> ADEEQVFHFYWLDAYEDQYNQPGVVFLFGKVWIESAETHVSCCVMVKNIERTLYFLPREMKIDLNTGKETGTPISMKDVYEEFDEKIATKYKIMKFKSKPVEKNYAFEIPDVPEKSEYLEVKYSAEMPQLPQDLKGETFSHVFGTNTSSLELFLMNRKIKGPCWLEVKSPQLLNQPVSWCKAEAMALKPDLVNVIKDVSPPPLVVMAFSMKTMQNAKNHQNEIIAMAALVHHSFALDKAAPKPPFQSHFCVVSKPKDCIFPYAFKEVIEKKNVKVEVAATERTLLGFFLAKVHKIDPDIIVGHNIYGFELEVLLQRINVCKAPHWSKIGRLKRSNMPKLGGRSGFGERNATCGRMICDVEISAKELIRCKSYHLSELVQQILKTERVVIPMENIQNMYSESSQLLYLLEHTWKDAKFILQIMCELNVLPLALQITNIAGNIMSRTLMGGRSERNEFLLLHAFYENNYIVPDKQIFRKPQQKLGDEDEEIDGDTNKYKKGRKKAAYAGGLVLDPKVGFYDKFILLLDFNSLYPSIIQEFNICFTTVQRVASEAQKVTEDGEQEQIPELPDPSLEMGILPREIRKLVERRKQVKQLMKQQDLNPDLILQYDIRQKALKLTANSMYGCLGFSYSRFYAKPLAALVTYKGREILMHTKEMVQKMNLEVIYGDTDSIMINTNSTNLEEVFKLGNKVKSEVNKLYKLLEIDIDGVFKSLLLLKKKKYAALVVEPTSDGNYVTKQELKGLDIVRRDWCDLAKDTGNFVIGQILSDQSRDTIVENIQKRLIEIGENVLNGSVPVSQFEINKALTKDPQDYPDKKSLPHVHVALWINSQGGRKVKAGDTVSYVICQDGSNLTASQRAYAPEQLQKQDNLTIDTQYYLAQQIHPVVARICEPIDGIDAVLIATWLGLDPTQFRVHHYHKDEENDALLGGPAQLTDEE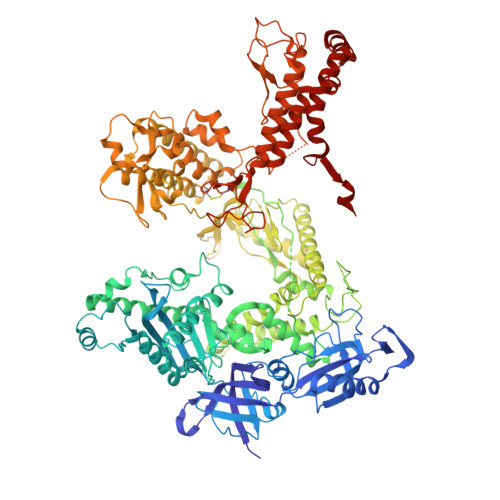KYRDCERFKCPCPTCGTENIYDNVFDGSGTDMEPSLYRCSNIDCKASPLTFTVQLSNKLIMDIRRFIKKYYDGWLICEEPTCRNRTRHLPLQFSRTGPLCPACMKATLQPEYSDKSLYTQLCFYRYIFDAECALEKLTTDHEKDKLKKQFFTPKVLQDYRKLKNTAEQFLSRSGYSEVNLSKLFAGCAVKS>MGSHHHHHHGSLKLMIKINEAVFYDRIT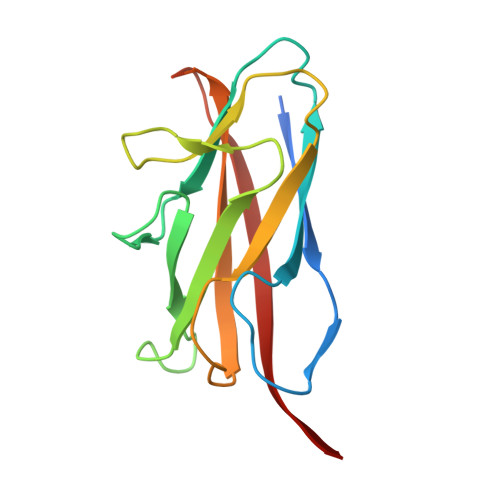SNKIIGTGHLFNREGKKILISSSLEKIKNTPGAYIIRGQNNSAHKLRIRIGGEDWQPDNSGIGMVSHSDFTNEFNIYFFGNGDIPVDTYLISIYATEIELDNKQGFVGNKAVVQAAVTIAAKLN[6x]>G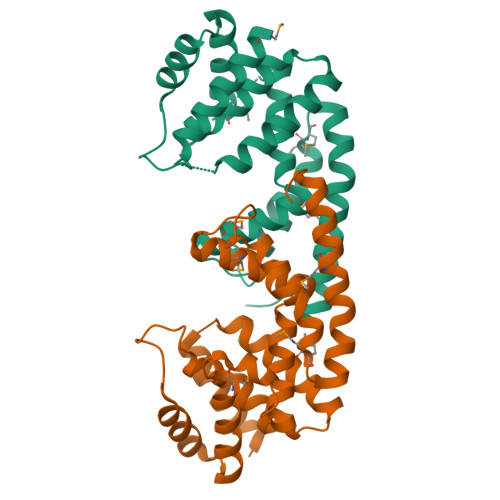SAKDPMTELKQADQIRTWVQSVLTGESSGHDWLHISRVADLAVYIGEKENADLFIVETAALVHDLIDVKLPDTIRLSVSEVYNQLVTFGIGKEDADRVIHIITKMSFRDREKLEGEPLSIEGKVVQDADRLDAIGAVGIARAFMFAGAKGHGLYGDDQSAYAHFFHKLLRLIDMMNTDTARELAEERHEFMLQYIRQLEKDIPGIDAKTS[2x]> G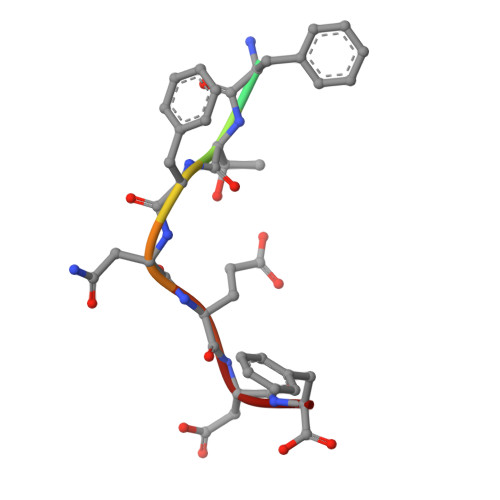AFTFNEDF> GSAMGNYMGNPWTEYMAKYDIEEVHGSGIRVDLGEDAEVAGTQYRLPSGKCPVFGKGIIIENSNTTFLTPVATGNQYLKDGGFAFPPTEPLMSPMTLDEMRHFYKDNKYVKNLDELTLCSRHAGNMIPDNDKNSNYKYPAVYDDKDKKCHILYIAAQENNGPRYCNKDESKRNSMFCFRPAKDISFQNYTYLSKNVVDNWEKVCPRKNLQNAKFGLWVDGNCEDIPHVNEFPAIDLFECNKLVFELSASDQPKQYEQHLTDYEKIKEGFKNKNASMIK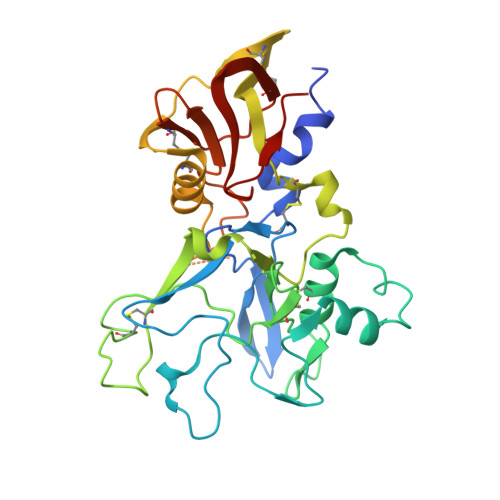SAFLPTGAFKADRYKSHGKGYNWGNYNTETQKCEIFNVKPTCLINNSSYIATTALSHPIEVEAAALVPR(3~{R},5~{R})-1-[2,4-bis(fluoranyl)phenyl]-5-oxidanyl-pyrrolidine-3-carboxylic acid | C11 H11 F2 N O3 | 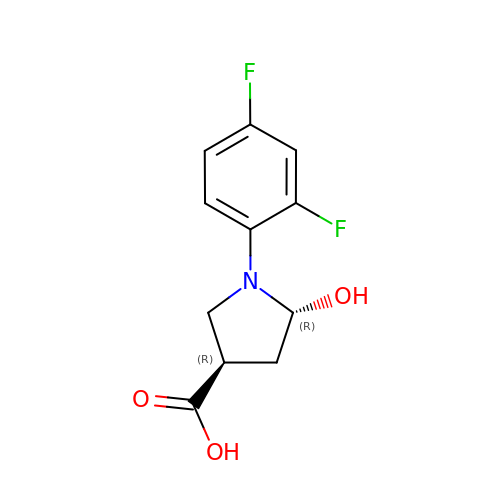HKKAZODAIOIPGM-LHLIQPBNSA-N> GLVPRGSHMMEILRGSPALSAFRINKLLARFQAANLQVHNIYAEYVHFADLNAPLNDSEQAQLTRLLQYGPALSSHTPAGKLLLVTPRPGTISPWSSKATDIAHNCGLQQVDRLERGVAYYIEASTLTAEQWRQVAAELHDRMMETVFSSLTDAEKLFIHHQPAPVSSVDLLGEGRQALIDANLRLGLALAEDEIDYLQEAFTKLGRNPNDIELYMFAQANSEHCRHKIFNADWIIDGKPQPKSLFKMIKNTFETTPDYVLSAYKDNAAVMEGSAVGRYFADHNTGRYDFHQEPAHILMKVETHNHPTAISPWPGAATGSGGEIRDEGATGRGAKPKAGLVGFSVSNLRIPGFEQPWEEDFGKPERIVTALDIMTEGPLGGAAFNNEFGRPALTGYFRTYEEKVNSHNGEELRGYHKPIMLAGGIGNIRADHVQKGEIVVGAKLIVLGGPAMNIGLGGGAASSMASGQSDAAADFASVQRDNPEMERRCQEVIDRCWQLGDANPILFIHDVGAGGLSNAMPELVSDGGRGGKFELRDILSDEPGMSPLEIWCNESQERYVLAVAADQLPLFDELCKRERAPYAVIGDATEEQHLSLHDNHFDNQPIDLPLDVLLGKTPKMTRDVQTLKAKGDALNRADITIADAVKRVLHLPTVAEKTFLVTIGDRTVTGMVARDQMVGPWQVPVADCAVTTASLDSYYGEAMSIGERAPVALLDFAASARLAVGEALTNIAATQIGDIKRIKLSANWMAAAGHPGEDAGLYDAVKAVGEELCPQLGLTIPVGKDSMSMKTRWQEGNEQREMTSPLSLVISAFARVEDVRHTLTPQLSTEDNALLLIDLGKGHNALGATALAQVYRQLGDKPADVRDV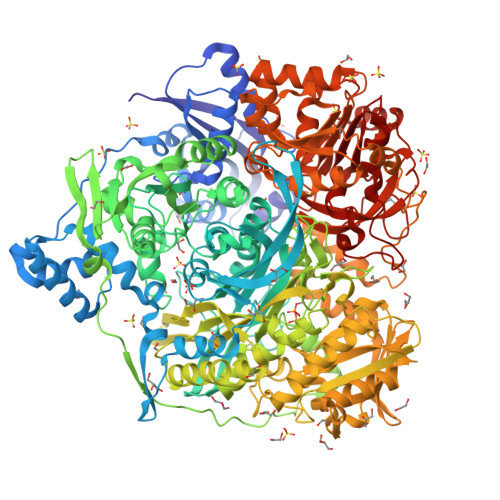AQLKGFYDAMQALVAARKLLAWHDRSDGGLLVTLAEMAFAGHCGVQVDIAALGDDHLAALFNEELGGVIQVRAEDRDAVEALLAQYGLADCVHYLGQALAGDRFVITANDQTVFSESRTTLRVWWAETTWQMQRLRDNPQCADQEHEAKANDTDPGLNVKLSFDINEDIAAPYIATGARPKVAVLREQGVNSHVEMAAAFHRAGFDAIDVHMSDLLGGRIGLGNFHALVACGGFSYGDVLGAGEGWAKSILFNHRVRDEFETFFHRPQTLALGVCNGCQMMSNLRELIPGSELWPRFVRNHSDRFEARFSLVEVTQSPSLLLQGMVGSQMPIAVSHGEGRVEVRDDAHLAALESKGLVALRYVDNFGKVTETYPANPNGSPNGITAVTTENGRVTIMMPHPERVFRTVANSWHPENWGEDSPWMRIFRNARKQLG> MNLVLMGLPGAGKGTQGERIVEDYGIPHISTGDMFRAAMKEETPLGLEAKSYIDKGELVPDEVTIG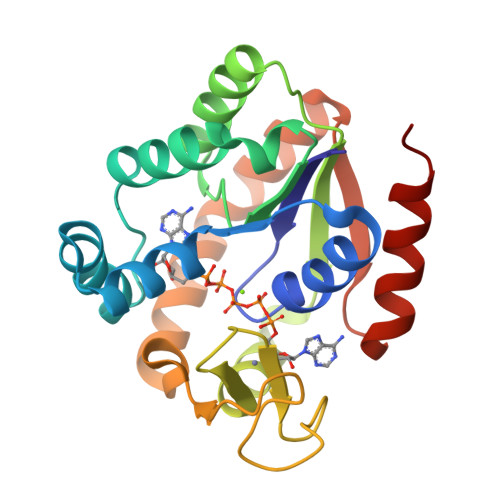IVKERLGKDDCERGFLLDGFPRTVAQAEALEEILEEYGKPIDYVINIEVDKDVLMERLTGRRICSVCGTTYHLVFNPPKTPGICDKDGGELYQRADDNEETVSKRLEVNMKQTQPLLDFYSEKGYLANVNGQRDIQDVYADVKDLLGRLKK> PGYLNDIPRHGMFVKDLILLVNDTAAVAYDPMENECYLTALAEQIPRNHSSIVTQQNQVYVVGGLYVDEE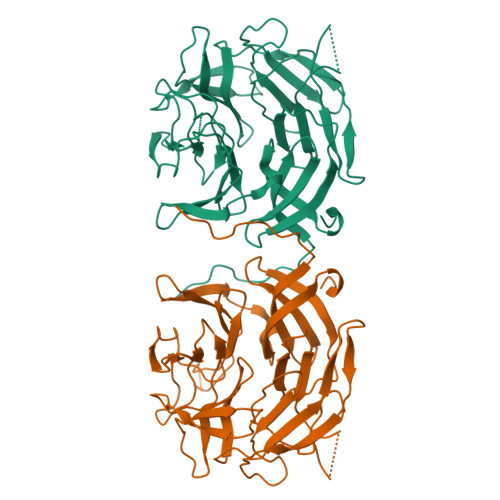NKDQPLQSYFFQLDNVSSEWVGLPPLPSARCLFGLGEVDDKIYVVAGKDLQTEASLDSVLCYDPVAAKWSEVKNLPIKVYGHNVISHNGMIYCLGGKTDDKKCTNRVFIYNPKKGDWKDLAPMKTPRSMFGVAIHKGKIVIAGGVTEDGLSASVEAFDLKTNKWEVMTEFPQERSSISLVSLAGSLYAIGGFAMIQLESKEFAPTEVNDIWKYEDDKKEWAGMLKEIRYASGASCLATRLNLFKLSKL> MASNYNSGLKIGAWVGTQPSESAIKSFQELQGRKL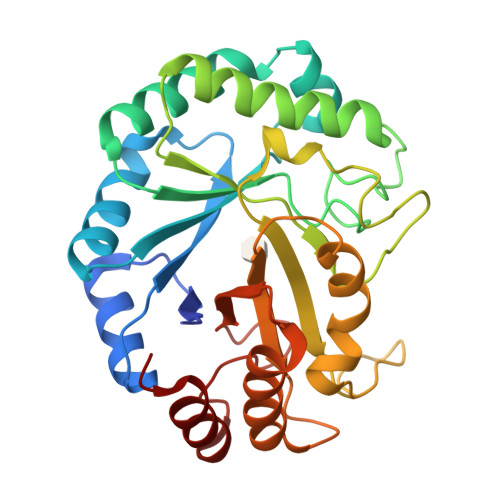DIVHQFINWSTDFSWVRPYADAVYNNGSILMITWEPWEYNTVDIKNGKADAYITRMAQDMKAYGKEIWLRPLHEANGDWYPWAIGYSSRVNTNETYIAAFRHIVDIFRANGATNVKWVFNVNCDNVGNGTSYLGHYPGDNYVDYTSIDGYNWGTTQSWGSQWQSFDQVFSRAYQALASINKPIIIAEFASAEIGGNKARWITEAYNSIRTSYNKVIAAVWFHENKETDWRINSSPEALAAYREAIGAL> TMCY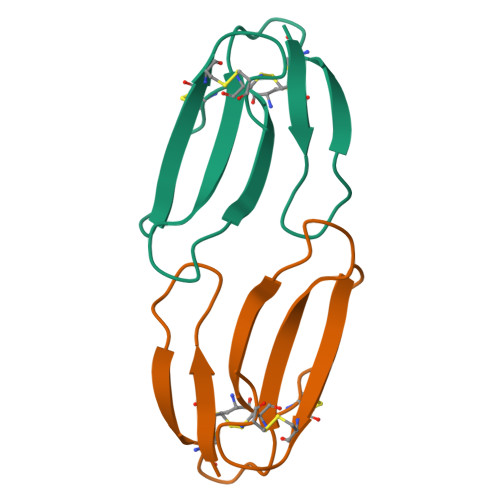SHTTTSRAILTNCPGETNCYKKSRRHPPKMVLGRGCGCPTVAPGIKLNCCTTDKCNY>MATNLRGVMAALLTPFDQQQALDKASLRRLVQFN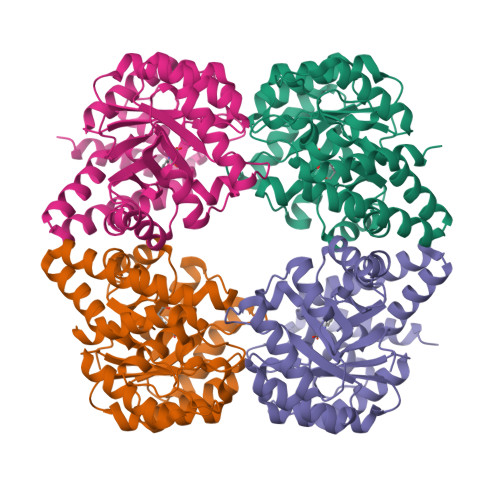IQQGIDGLYVGGSTGEAFVQSLSEREQVLEIVAEEAKGKIKLIAHVGCVSTAESQQLAASAKRYGFDAVSAVTPFYYPFSFEEHCDHYRAIIDSADGLPMVVYNIPARSGVKLTLDQINTLVTLPGVGALKQTSGDLYQMEQIRREHPDLVLYNGYDEIFASGLLAGADGGIGSTYNIMGWRYQGIVKALKEGDIQTAQKLQTECNKVIDLLIKTGVFRGLKTVLHYMDVVSVPLCRKPFGPVDEKYLPELKALAQQLMQERG[4x]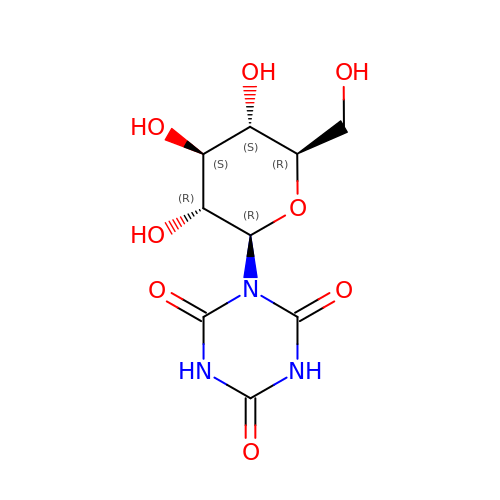1-beta-D-glucopyranosyl-1,3,5-triazinane-2,4,6-trione | C9 H13 N3 O8 | AWNGSFAGXKOIML-VFUOTHLCSA-N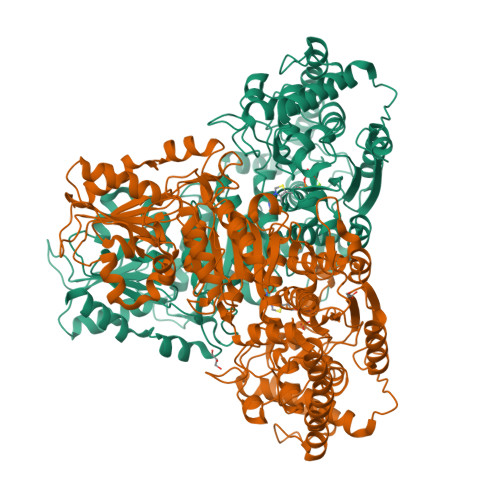>MTTLEEISALTRPRHPDYWTEIDSAAVDTIRVLAADAVQKVGNGHPGTAMSLAPLAYTLFQRTMRHDPSDTHWLGRDRFVLSAGHSSLTLYIQLYLGGFGLELSDIESLRTWGSKTPGHPEFRHTPGVEITTGPLGQGLASAVGMAMASRYERGLFDPDAEPGASPFDHYIYVIASDGDIEEGVTSEASSLAAVQQLGNLIVFYDRNQISIEDDTNIALCEDTAARYRAYGWHVQEVEGGENVVGIEEAIANAQAVTDRPSFIALRTVIGYPAPNLMDTGKAHGAALGDDEVAAVKKIVGFDPDKTFQVREDVLTHTRGLVARGKQAHERWQLEFDAWARREPERKALLDRLLAQKLPDGWDADLPHWEPGSKALATRAASGAVLSALGPKLPELWGGSADLAGSNNTTIKGADSFGPPSISTKEYTAHWYGRTLHFGVREHAMGAILSGIVLHGPTRAYGGTFLQFSDYMRPAVRLAALMDIDTIYVWTHDSIGLGEDGPTHQPIEHLSALRAIPRLSVVRPADANETAYAWRTILARRNGSGPVGLILTRQGVPVLDGTDAEGVARGGYVLSDAGGLQPGEEPDVILIATGSEVQLAVAAQTLLADNDILARVVSMPCLEWFEAQPYEYRDAVLPPTVSARVAVEAGVAQCWHQLVGDTGEIVSIEHYGESADHKTLFREYGFTAEAVAAAAERALDN[4x]> GSASKKLPPKFYERATSNKTQRVVSVCKMYFLEHYCDMFDYVISRRQRTKQVLEYLQQQSQLPNSDQIKLNEEWSSYLQREHQVLRKRRLK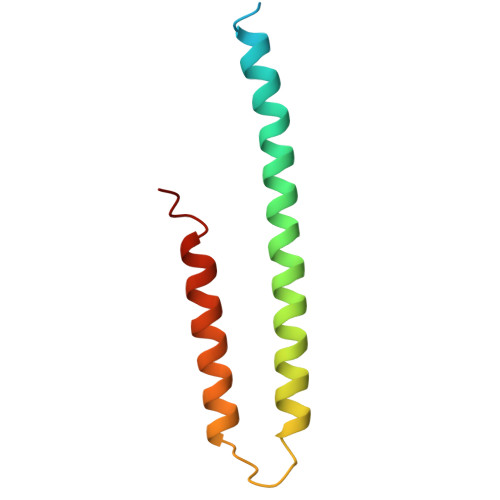PK>SNAMRQSGSWMTIWDDRILEIIHEEGNGSPKELEDRDEIRISKSSVSRRLKKLADHDLLQPLANGVYVITEEGEAYLNGEYDAGKER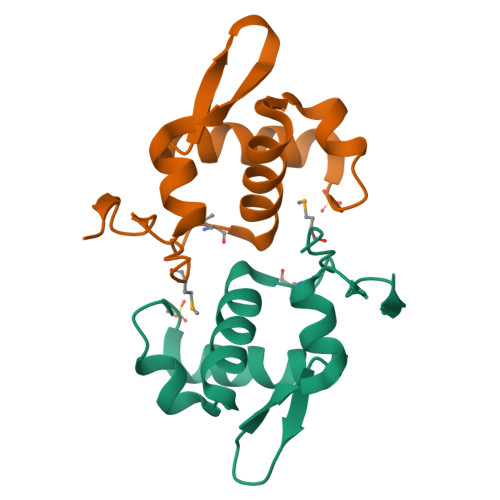YINRGNSTDEENGADAPDGPGINS[2x]>GRFSFSPEPTLEDIRRLHAEFAAERDWEQFHQPRNLLLALVGEVGELAELFQWKTDGEPGPQGWSPRERAALQEELSDVLIYLVALAARCRVDLPLAVLSKMDINR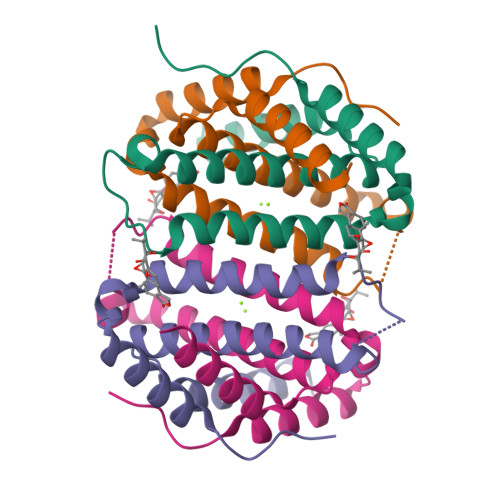RRYP[8x]>[2x]MRKKISIIGAGFVGSTTAHWLAAKELGDIVLLDIVEGVPQGKALDLYEASPIEGFDVRVTGTNNYADTANSDVIVVTSGAPRKPGMSREDLIKVNADITRACISQAAPLSPNAVIIMVNNPLD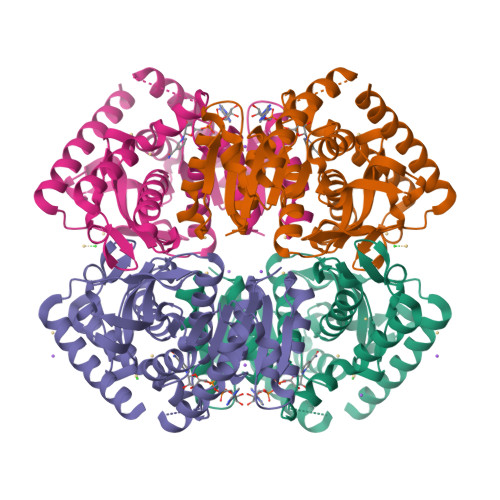AMTYLAAEVSGFPKERVIGQAGVLDAARYRTFIAMEAGVSVQDVQAMLMGGHGDEMVPLPRFSTISGIPVSEFIAPDRLAQIVERTRKGGGEIVNLLKTGSAYYAPAAATAQMVEAVLKDKKRVMPVAAYLTGQYGLNDIYFGVPVILGAGGVEKILELPLNEEEMALLNASAKAVRATLDTLKSL>[4x]MKHHHHHHPMASAATESATATATLEETL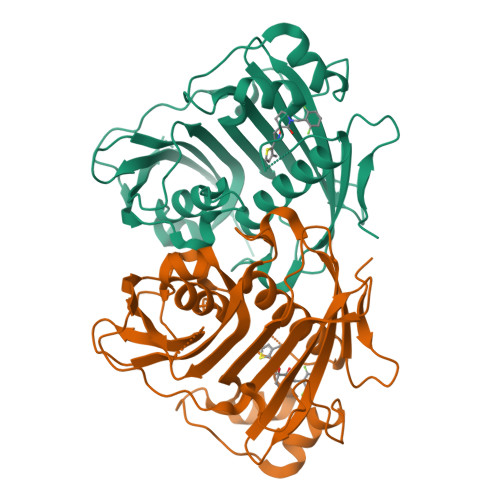AQRLRLGSLEPDGLSYKESFIVRSYEVGVNKTATVETIANLLQEVGCNHAQSVGFSTDGFATTTTMRLLRLIWVTARMHIEIYKYPAWGDVVEIETWCQEDGKIGTRRDWIIKDYSTGVVIGRATSKWVMMNQDTRRLQRVNDEVREEYLIFCPRTPRLAFPEEDSDSLKKIPKLEEPAQSSKLGLVPRRADLDMNQHVNNVTYIGWVLESIPQEIIDTHELQTITLDYRRECQHDDIVDSLSSREFGDTPQNGNHSTGRKEGECQFLHFLKLSGSGLEINRGRTQWRRLAK> MVLLVIGLPLVSLVVALVAAAAPDSQVCDVDSTATCKITATPSQFQPALLNASKWIWTGENPIPGGSNIISTRPFRKNITAPCGKCSVCATIVVASDDAHTFYVNGVRIGTGAGFRQGQALFVALQPTWNLFAIAGQNLVANSPAGIMASILVHFSDGTSETFVTDESWKTLRAAPPENFQLPSTNDSNWPSAAVQGAYQNSVWGPPVLPPVLPLRGS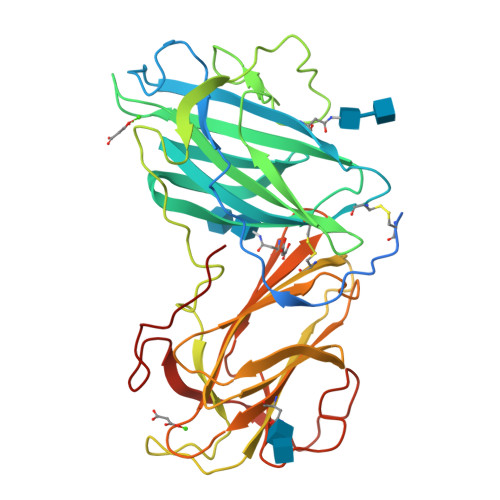NWIWTSDNVNGAAPVGSRAFRKTVNQCTKVAVCATVLIAADDRYTLYVNGATVGSGSSYTVADAYTIPNLHPTFNTFAINATNGGGPAGVIATILITYSDGSNETVVTDASWKAIQTIPQGFQPPLIDEFGWESAKIIGAFGVAPWGAGMVIPSA> GSMPAIMTMLADHAARQLLDFSQKLDINLLDNVVNCLYHGEGAQQRM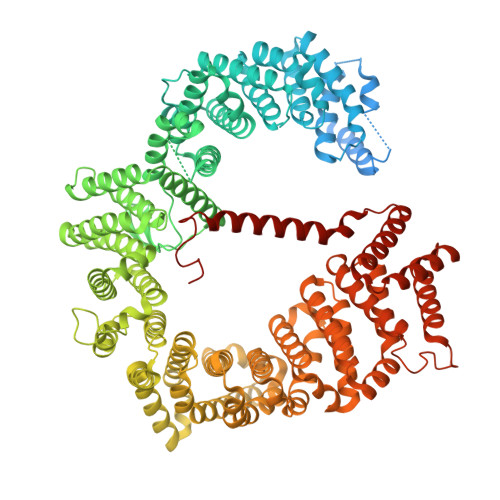AQEVLTHLKEHPDAWTRVDTILEFSQNMNTKYYGLQILENVIKTRWKILPRNQCEGIKKYVVGLIIKTSSDPTCVEKEKVYIGKLNMILVQILKQEWPKHWPTFISDIVGASRTSESLCQNNMVILKLLSEEVFDFSSGQITQVKSKHLKDSMCNEFSQIFQLCQFVMENSQNAPLVHATLETLLRFLNWIPLGYIFETKLISTLIYKFLNVPMFRNVSLKCLTEIAGVSVSQYEEQFVTLFTLTMMQLKQMLPLNTNIRLAYSNGKDDEQNFIQNLSLFLCTFLKEHDQLIEKRLNLRETLMEALHYMLLVSEVEETEIFKICLEYWNHLAAELYRESPFSTSASPLLSGSQHFDVPPRRQLYLPMLFKVRLLMVSRMAKPEEVLVVENDQGEVVREFMKDTDSINLYKNMRETLVYLTHLDYVDTERIMTEKLHNQVNGTEWSWKNLNTLCWAIGSISGAMHEEDEKRFLVTVIKDLLGLCEQKRGKDNKAIIASNIMYIVGQYPRFLRAHWKFLKTVVNKLFEFMHETHDGVQDMACDTFIKIAQKCRRHFVQVQVGEVMPFIDEILNNINTIICDLQPQQVHTFYEAVGYMIGAQTDQTVQEHLIEKYMLLPNQVWDSIIQQATKNVDILKDPETVKQLGSILKTNVRACKAVGHPFVIQLGRIYLDMLNVYKCLSENISAAIQANGEMVTKQPLIRSMRTVKRETLKLISGWVSRSNDPQMVAENFVPPLLDAVLIDYQRNVPAAREPEVLSTMAIIVNKLGGHITAEIPQIFDAVFECTLNMINKDFEEYPEHRTNFFLLLQAVNSHCFPAFLAIPPTQFKLVLDSIIWAFKHTMRNVADTGLQILFTLLQNVAQEEAAAQSFYQTYFCDILQHIFSVVTDTSHTAGLTMHASILAYMFNLVEEGKISTSLNPGNPVNNQIFLQEYVANLLKSAFPHLQDAQVKLFVTGLFSLNQDIPAFKEHLRDFLVQIKEFAGEDTSDLFLEEREIALRQADEEKHKRQMSVPGIFNPHEIPEEMCD> GSMVEATAQETDRPRFSFSIAAREGKARTGTIEMKRGVIRTPAFMPVGTAATVKALKPETVRATGADIILGNTYHLMLRPGAERIAKLGGLHSFMGWDRPILTDSGGYQVMSLSSLTKQSEEGVTFKSHLDGSRHMLSPERSIEIQHLLGSDIVMAFDECTPYPATPSRAASSMERSMRWAKRSRDAFDSRKEQAENAALFGIQQGSVFENLRQQSADALAEIGFDGYAVGGLAVGEGQDEMFRVLDFSVPMLPDDKPHYLMGVGKPDDIVGAVERGIDMFDCVLPTRSGRNGQAFTWDGPINIRNARFSEDLKPLDSECHCAVCQKWSRAFIHHLIRAGEILGAMLMTEHNIAFYQQLMQKIRDSIS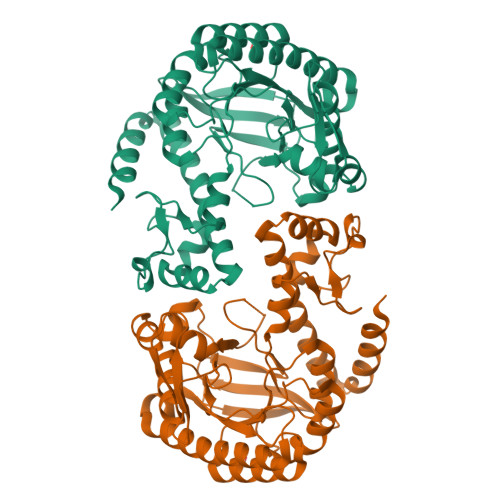EGRFSQFAQDFRARYFARNS In mammals, the canonical Hippo pathway contains a core kinase cascade, formed by STE20-like MST1/2 kinases, Large Tumor Suppressor LATS1/2 kinases, the WW-domain containing scaffold protein Salvador (SAV1) and the adaptor protein MOB1. MST1/2 contain an N-terminal kinase domain and a C-terminal coiled-coil SARAH domain, which are separated by a flexible linker. MST1 and MST2 can each form a constitutive homodimer through the SARAH domain, and kinase activation is achieved by trans-autophosphorylation of the activation loop (T183 for MST1 and T180 for MST2). In this study, using a combination of biochemical, structural, and cell biological experiments, we establish the PP2A complex, STRIPAKSLMAP, as a key negative regulator of Hippo signaling in human cells, and show that SAV1 promotes MST1/2 activation through antagonizing the STRIPAKSLMAP PP2A phosphatase activity.

A proteomic study has shown that MST1/2 interact with a specific PP2A complex called STRIPAK through the N-terminal forkhead associated (FHA) domain of the adaptor protein SLMAP. FHA domains are specific phospho-threonine (pT) binding modules. Like other FHA domains, SLMAP FHA adopts a typical β sandwich fold that consists of two large β sheets. One sheet contains six antiparallel strands: β2, β1, β11, β10, β7, and β8, while the other sheet contains five mixed parallel/antiparallel strands: β4, β3, β5, β6, and β9. The major structural differences between SLMAP FHA and other FHAs with known structures reside in the loops connecting the β strands, especially the long loop between β10 and β11, which forms a short β1’/β2’ hairpin and protrudes away from the FHA core. Despite the differences of the loops at the pT binding site among various FHA domains, the pT-binding residues, R32, S52 and H55, can be structurally overlaid with the corresponding residues from other FHAs, suggesting that the mode of pT recognition is highly conserved among FHA domains.

> MPSALAIFTCRPNSHPFQERHVYLDEPIKIGRSVARCRPAQNNATFDCKVLSRNHALVWFDHKTGKFYLQDTKSSNGTFINSQRLSRGSEESPPCEILSGDIIQFGVDVTENTRKVTHGCIVSTIKLFLPDGMEARLRSD> KATMQCGENEKYDSCGSKECDKKCKYDGVEEEDDEEPNVPCLVRVCHQDCVCEEGFYRNKDDKCVSAEDCE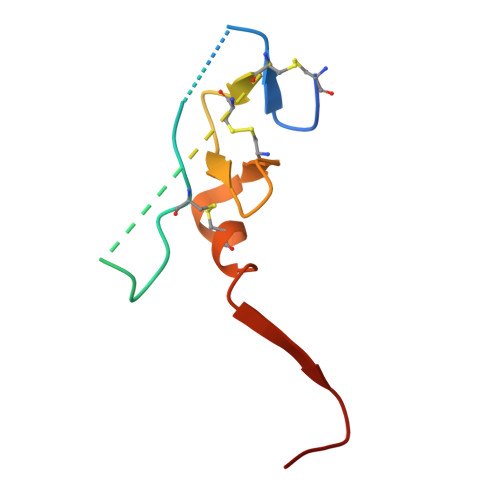LDNMDFIYPGTRN>[4x]MVKSSGTERKERMDTSSLMEQILSNDNLNRAYLQVVRNKGAEGVDGMKYTELKEYLAKNGEIIKEQLRIRKYKPQPVRRVEIPKPDGGVRNLGVPTVTDRFIQQAIAQVLTPIYEEQFHDHSYGFRPNRCAQQAILTALDMMNDGNDWIVDIDLEKFFDTVNHDKLMTIIGRTIKDGDVISIVRKYLVSGIMIDDEYEDSIVGTPQGGNLSPLLANIMLNELDK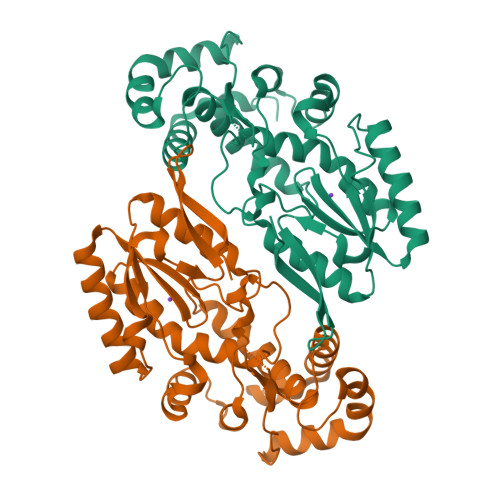EMEKRGLNFVRYADDCIIMVGSEMSANRVMRNISRFIEEKLGLKVNMTKSKVDRPRGIKYLGFGFYYDTSAQQFKAKPHAK>MAEDKSKRDSIEMSMKGCQTNNGFVHNEDILEQTPDPGSSTDNLKHSTRGILGSQEPDFKGVQPYAGMPKEVLFQFSGQARYRIPREILFWLTVASVLVLIAATIAIIALSPKCLDWWQEGPMYQIYPRSFKDSNKDGNGDLKGIQDKLDYITALNIKTVWITSFYKSSLKDFRYGVEDFREVDPIFGTMEDFENLVAAIHDKGLKLIIDFIPNHTSDKHIWFQLSRTRTGKYTDYYIWHDCTHENGKTIPPNNWLSVYGNSSWHFDEVRNQCYFHQFMKEQPDLNFRNPDVQEEIKEILRFWLTKGVDGFSLDAVKFLLEAKHLRDEIQVNKTQIPDTVTQYSELYHDFTTTQVGMHDIVRSFRQTMDQYSTEPGRYRFMGTEAYAESIDRTVMYYGLPFIQEADFPFNNYLSMLDTVSGNSVYEVITSWMENMPEGKWPNWMIGGPDSSRLTSRLGNQYVNVMNMLLFTLPGTPITYYGEEIGMGNIVAANLNESYDINTLRSKSPMQWDNSSNAGFSEASNTWLPTNSDYHTVNVDVQKTQPRSALKLYQDLSLLHANELLLNRGWFCHLRNDSHYVVYTRELDGIDRIFIVVLNFGESTLLNLHNMISGLPAKMRIRLSTNSA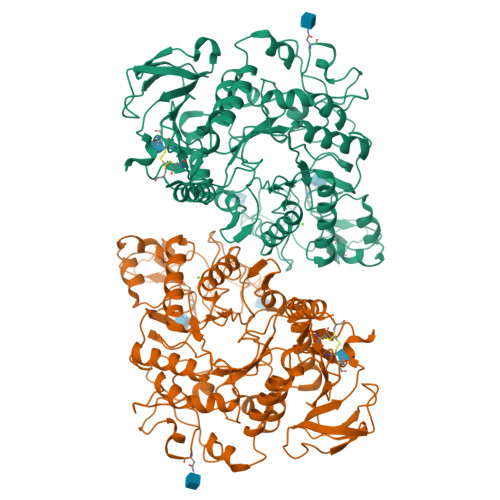DKGSKVDTSGIFLDKGEGLIFEHNTKNLLHRQTAFRDRCFVSNRACYSSVLNILYTSC[2x]>CGCT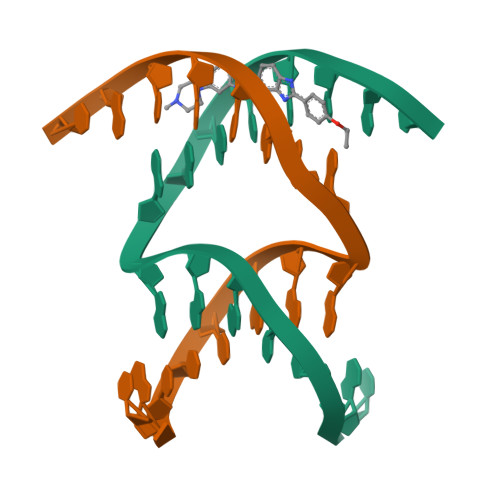TAAGGAATTCGC[2x]> MVPISPIETVPVKLKPGMDGPKVKQWPLTEEKIKALVEICTEMEKEGKISKIGPENPYNTPVFAIKKKDSTKWRKLVDFRELNKRTQDFWEVQLGIPHPAGLKKKKSVTVLDVGDAYFSVPLDEDFRKYTAFTIPSINNETPGIRYQYNVLPQGWKGSPAIFQSSMTKILEPFKKQNPDIVIYQYMDDLYVGSDLEIGQHRTKIEELRQHLLRWGLTTPDKKHQKEPPFLWMGYELHPDKWTVQPIVLPEKDSWTVNDIQKLVGKLNWASQIYPGIKVRQLSKLLRGTKALTEVIPLTEEAELELAENREILKEPVHGVYYDPSKDLIAEIQKQGQGQWTYQIYQEPFKNLKTGKYARMRGAHTNDVKQLTEAVQKITTESIVIWGKTPKFKLPIQKETWETWWTEYWQATWIPEWEFVNTPPLVKLWYQLEKEPIVGAETFYVDGAANRETKLGKAGYVTNKGRQKVVPLTNTTNQKTELQAIYLALQDSGLEVNIVTDSQYALGIIQAQPDKSESELVNQIIEQLIKKEKVYLAWVP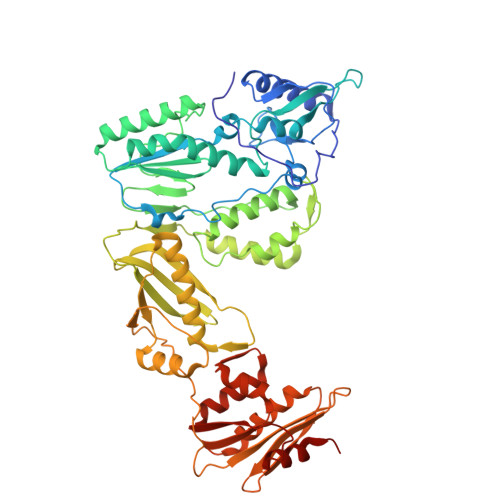AHKGIGGNEQVDKLVSAG> GHMDSTTIQQNKDTLSQIVVFPTGNYDKNEANAMVNRLANIDGKYLNALKQNNLKIKLLSGKLTDEKEYAYLKGVVPKGWEGTGKTWDDVPGLGGSTVALRIGFSNKGKGHDAINLELHATAHAIDHIVLNDISKSAQFKQIFAKEGRSLGNVNFLGVYPE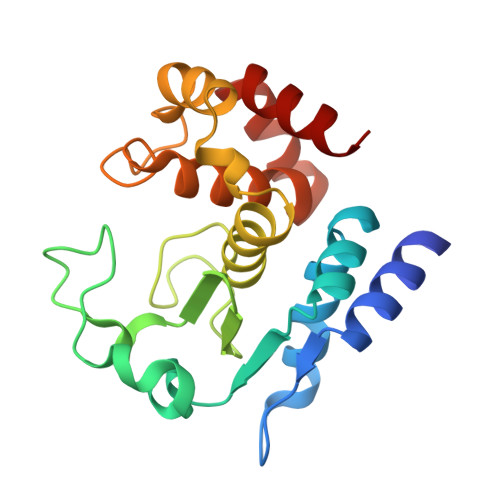EFFAESFAYYYLNQDTNSKLKSACPQTYSFLQNLAK> STDNAETGVIEAGNTDTDFSGELAAPGSNHTNVKFLFDRSRLLNVIKVLEKDAVFPRPFPTQEGAQQDDGYFCLLTPRPTVASRPATRFGLYANPSGSGVLANTSLDFNFYSLACFTYFRSDLEVTVVSLEPDLEFAVGWFPSGSEYQASSFVYDQLHVPFH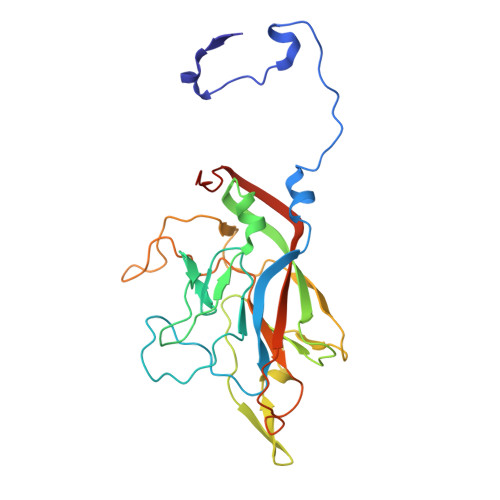FTGRTPRAFASKGGKVSFVLPWNSVSSVLPVRWGGASKLSSATRGLPAHADWGTIYAFVPRPNEKKSTAVKHVAVYIRYKNARAWCPSMLPFRSYKQKMLM>[6x]MAMWTPQTGKLYLPPTTPVAKVQSTDEYVYPTSLFCHAHTDRLLTVGHPFFSVIDNDKVTVPKVSGNQYRVFRLKFPDPNKFALPQKDFYDPEKERLVWRLRGLEIGRGGPLGIGTTGHPLFNKLGDTENPNKYQQGSKDNRQNTSMDPKQTQLFIVGCEPPTGEHWDVAKPCGALEKGDCPPIQLVNSVIEDGDMCDIGFGNMNFKELQQDRSGVPLDIVSTRCKWPDFLKMTNEAYGDKMFFFGRREQVYARHFFTRNGSVGEPIPNSVSPSDFYYAPDSTQDQKTLAPSVYFGTPSGSLVSSDGQLFNRPFWLQRAQGNNNGVCWHNELFVTVVDNTRNTNFTISQQTNTPNPDTYDSTNFKNYLRHVEQFELSLIAQLCKVPLDPGVLAHINTMNPTILENWNLGFVPPPQQSISDDYRYITSSATRCPDQNPPKEREDPYKGLIFWEVDLTERFSQDLDQFALGRKFLYQAGIRTAVTGRGVKRAASTTSASSRRVVKRKRGSK

Papillomavirus is a T = 7d icosahedral, double stranded DNA virus with a genome of ~8 kb. The capsid is composed of 72 capsomers, each containing five copies of L1, the major capsid protein. For each copy of L1 a loop of the C-terminus forms a connecting arm by extending to a neighboring capsomer, forming a stabilizing disulfide bond, and returning to the donating capsomer. The secondary structure of L1 proteins take the form of the ubiquitous β-jellyroll made up of eight anti-parallel β-strands (BIDG and CHEF) with loop regions that extend outward from the surface of the capsid and constitute the majority of the L1 hypervariable regions.

Here, we purified a native mouse papillomavirus (MmuPV1), for which we have used ISECC to obtain high resolution maps and made a comparison for the first time between native papillomavirus and lab generated capsids. The subparticle refinements were recombined into an icosahedral capsid with 3.3 Å resolution overall (ISECC_Recombine), a dramatic improvement over the original 4.4 Å map. The high resolution of the recombined map allowed for the full asymmetric unit of MmuPV1 to be built for the first time. The L1 protein structure was reliably visualized from Thr16–Ala481. The build of the L1 protein revealed the typical papillomavirus secondary structure elements of BIDG and CHEF anti-parallel beta strands making up the L1 core within each capsomer. Despite the sequence deviation between HPV and MmuPV1 (53% identity) there is structural conservation of the secondary, tertiary, and quaternary structures. Each copy of L1 has a C-terminal loop region spanning Trp 406–Trp 451 and five of these connecting arms extend from each capsomer, independent of whether the capsomer is in the hexavalent or pentavalent icosahedral environment. Each of these loop regions extends to interact with a neighboring capsomer and these interactions are stabilized by a disulfide bond between Cys 432 of the connecting arm and Cys 173 of the neighboring capsomer. Despite each copy of L1 being chemically identical, there are six unique disulfide bonds that occur, one per L1 chain comprising the asymmetric unit. The resolution of the map density for the connecting arms ranged from 3.3–3.8 Å with some spots of weak density suggesting that the connecting arms are flexible.> IVLEPIYWNSSNSKFLPGQGLVLYPQIGDKLDIICPKVDSKTVGQYEYYKVYMVDK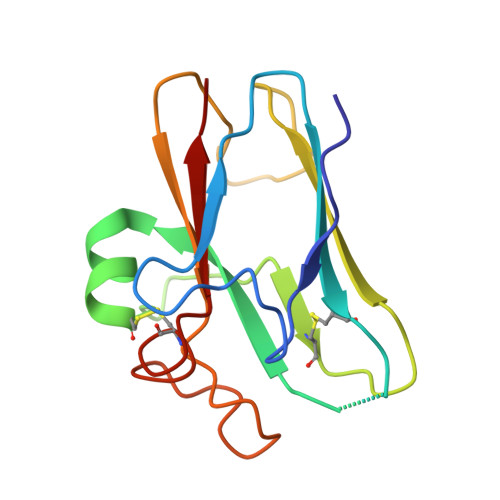DQADRCTIKKENTPLLNCAKPDQDIKFTIKFQEFSPNLWGLEFQKNKDYYIISTSNGSLEGLDNQEGGVCQTRAMKILMKVG> 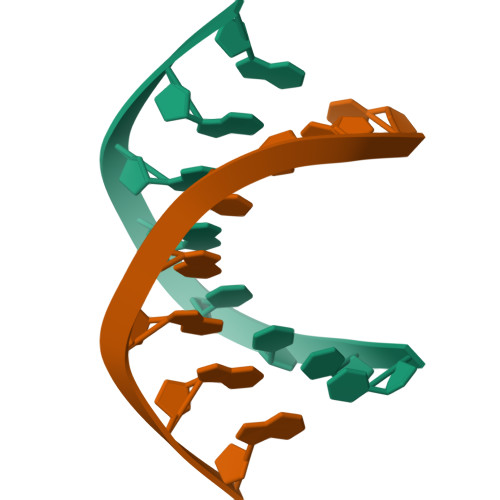CCCTAGGG>[2x]MADYKDDDDKSGRMPHFTVTKVEDPEEGAAASISQEPSLADIKARIQDSDEPDLSQNSITGEHSQLLDDGHKKARNAYLNNSNYEEGDEYFDKNLALFEEEMDTRPKVSSLLNRMANYTNLTQGAKEHEEAENITEGKKKPTKTPQMGTFMGVYLPCLQNIFGVILFLRLTWVVGTAGVLQAFAIVLICCCCTMLTAISMSAIATNGVVPAGGSYFMISRALGPEFGGAVGLCFYLGTTFAAAMYILGAIEIFLVYIVPRAAIFHSDDALKESAAMLNNMRVYGTAFLVLMVLVVFIGVRYVNKFASLFLACVIVSILAIYAGAIKSSFAPPHFPVCMLGNRTLSSRHIDVCSKTKEINNMTVPSKLWGFFCNSSQFFNATCDEYFVHNNVTSIQGIPGLASGIITENLWSNYLPKGEIIEKPSAKSSDVLGSLNHEYVLVDITTSFTLLVGIFFPSVTGIMAGSNRSGDLKDAQKSIPIGTILAILTTSFVYLSNVVLFGACIEGVVLRDKFGDAVKGNLVVGTLSWPSPWVIVIGSFFSTCGAGLQSLTGAPRLLQAIAKDNIIPFLRVFGHSKANGEPTWALLLTAAIAELGILIASLDLVAPILSMFFLMCYLFVNLACALQTLLRTPNWRPRFRYYHWALSFMGMSICLALMFISSWYYAIVAMVIAGMIYKYIEYQGAEKEWGDGIRGLSLSAARFALLRLEEGPPHTKNWRPQLLVLLKLDEDLHVKHPRLLTFASQLKAGKGLTIVGSVIVGNFLENYGEALAAEQTIKHLMEAEKVKGFCQLVVAAKLREGISHLIQSCGLGGMKHNTVVMGWPNGWRQSEDARAWKTFIGTVRVTTAAHLALLVAKNISFFPSNVEQFSEGNIDVWWIVHDGGMLMLLPFLLKQHKVWRKCSIRIFTVAQLEDNSIQMKKDLATFLYHLRIEAEVEVVEMHDSDISAYTYERTLMMEQRSQMLRHMRLSKTERDREAQLVKDRNSMLRLTSIGSDEDEETETYQEKVHMTWTKDKYMASRGQKAKSMEGFQDLLNMRPDQSNVRRMHTAVKLNEVIVNKSHEAKLVLLNMPGPPRNPEGDENYMEFLEVLTEGLERVLLVRGGGSEVITIYS

The electroneutral K+-Cl− cotransporters (KCCs) play fundamental roles in trans-epithelial transport, cell volume regulation, and neuronal excitability. The neuronal-specific KCC2 (SLC12A5) and glial-expressed KCC3 (SLC12A6) are essential for normal development and function of the nervous system. Here, we present single particle cryo-electron microscopy (cryo-EM) structures of the full-length human KCC2 and KCC3 at overall resolution of 3.2 and 3.3 Å, respectively. The structures of KCC2 and KCC3 are very similar to each other.

For simplicity, we mainly focused on KCC3 for structural analysis. KCC3 exists as a dimer in domain-swapping conformation. The TM domain and CTD are connected through a pair of scissor helices, which separate the two TM domains from different protomers resulting in a unique “Central Cleft” between TM domains at the cytosolic side. The extracellular domain (ECD) of the two protomers are placed in distance. Both TM domains, scissor helices and CTD are involved in dimerization of the transporter. The TM domain of KCC3 is captured in an inward-facing conformation, sharing the LeuT-fold as the members of the amino acids, polyamines and organocations (APC) superfamily, with TMs 3–5 and 8–10 forming the scaffold domain and TMs 1, 2, 6 and 7 constituting the bundle domain. A marked difference is observed in the C-terminal domain (CTD) compared with Danio rerio Na+-K+ Cl− cotransporter 1 (DrNKCC1), which rotates ~70° clockwise as seen from cytosolic side when transmembrane (TM) domains aligned together. A unique “L” shape N-terminal loop (residues N100–N120) is bound to the entry of the cytosolic vestibule of the transporter, which can be divided into an N lobe and a C lobe. The C lobe, which extends along TM8 and approaches CTD, is stabilized through salt bridges E116-K549 and E119-R886, as well as hydrophilic interaction between H115 and F203 from IL23. The binding locks the transporter in inward-facing state, prohibits the conformation change of the transporter.>KVEIIRGDHPEVYDDSAENEVPTAASIQRKAILETLTNLMLESQTPGTRQIREEESTIPIFAESTTQKTISVSDLPNNCLNASSLKCEIKGISTY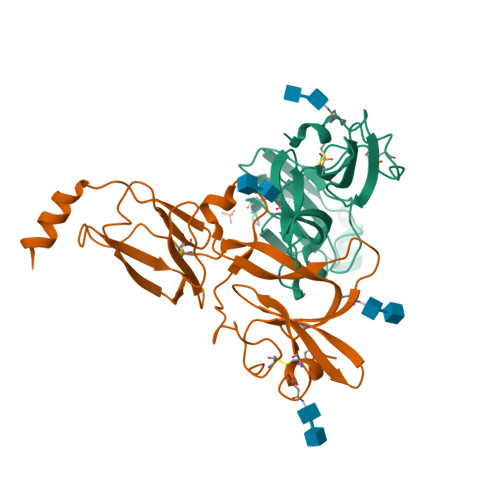NVYYQVENNGVIYSCVSDSAEGLEKCDNSLNLPKRFSKVPVIPITKLDNKRHFSVGTKFFISESLTQDNYPITYNSYPTNGTVSLQTVKLSGDCKITKSNFANPYTVSITSPEKIMGYLIKKPGENVEHKVISFSGSASITFTEEMLDGEHNLLCGDKSAKIPKTNKRVRDCIIKYSKSIYKQTACINF[4x]>[3x]MTKRVRLSDSFNPVYPYEDESTSQHPFINPGFISPNGFTQSPNGVLTLKCLTPLTTTGGSLQLKVGGGLTVDDTNGFLKENI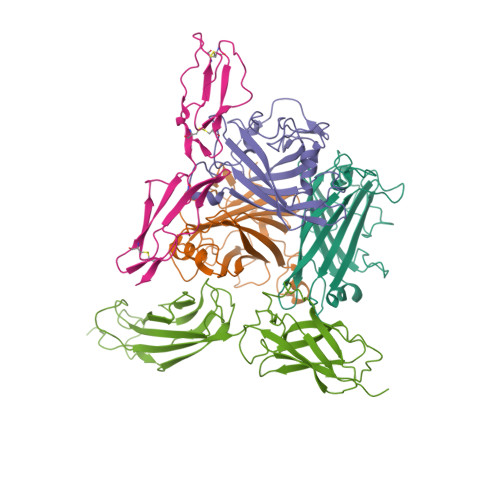SATTPLVKTGHSIGLPLGAGLGTNENKLCIKLGQGLTFNSNNICIDDNINTLWTGVNPTEANCQIMNSSESNDCKLILTLVKTGALVTAFVYVIGVSNNFNMLTTHRNINFTAELFFDSTGNLLTRLSSLKTPLNHKSGQNMATGAITNAKGFMPSTTAYPFNDNSREKENYIYGTCYYTASDRTAFPIDISVMLNRRAINDETSYCIRITWSWNTGDAPEVQTSATTLVTSPFTFYYIREDD;> MARSPGRAYALLLLLICFNVGSGLHLQVLSTRNENKLLPKHPHLVRQKRAWITAPVALREGEDLSKKNPIAKIHSDLAEERGLKITYKYTGKGITEPPFGIFVFNKDTGELNVTSILDREETPFFLLTGYALDARGNNVEKPLELRIKVLDINDNEPVFTQDVFVGSVEELSAAHTLVMKINATDADEPNTLNSKISYRIVSLEPAYPPVFYLNKDTGEIYTTSVTLDREEHSSYTLTVEARDGNGEVTDKPVKQAQVQIRILDVNDNIPVVENKVLEGMVEENQVNVEVTRIKVFDADEIGSDNWLANFTFASGNEGGYFHIETDAQTNEGIVTLIKEVDYEEMKNLDFSVIVANKAAFHKSIRSKYKPTPIPIKVKVKNVKEGIHFKSSVISIYVSESMDRSSKGQIIGNFQAFDEDTGLPAHARYVKLEDRDNWISVDSVTSEIKLAKLPDFESRYVQNGTYTVKIVAISEDYPRKTITGTVLINVEDINDNCPTLIEPVQTICHDAEYVNVTAEDLDGHPNSGPFSFSVIDKPPGMAEKWKIARQESTSVLLQQSEKKLGRSEIQFLISDNQGFSCPEKQVLTLTVCECLHGSGCREAQHDSYVGLGPAAIALMILAFLLLLLVPLLLLMCHCGKGAKGFTPIPGTIEMLHPWNNEGAPPEDKVVPSFLPVDQGGSLVGRNGVGGMAKEATMKGSSSASIVKGQHEMSEMDGRWEEHRSLLSGRATQFTGATGAIMTTETTKTARATGASRDMAGAQAAAVALNEEFLRNYFTDKAASYTEEDENHTAKDCLLVYSQEETESLNASIGCCSFIEGELDDRFLDDLGLKFKTLAEVCLGQKIDINKEIEQRQKPATETSMNTASHSLCEQTMVNSENTYSSGSSFPVPKSLQEANAEKVTQEIVTERSVSSRQAQKVATPLPDPMASRNVIATETSYVTGSTMPPTTVILGPSQPQSLIVTERVYAPASTLVDQPYANEGTVVVTERVIQPHGGGSNPLEGTQHLQDVPYVMVRERESFLAPSSGVQPTLAMPNIAVGQNVTVTERVLAPASTLQSSYQIPTENSMTARNTTVSGAGVPGPLPDFGLEESGHSNSTITTSSTRVTKHSTVQHSYS;> MEPPGRRECPFPSWRFPGLLLAAMVLLLYSFSDACEEPPTFEAMELIGKPKPYYEIGERVDYKCKKGYFYIPPLATHTICDRNHTWLPVSDDACYRETCPYIRDPLNGQAVPANGTYEFGYQMHFICNEGYYLIGEEILYCELKGSVAIWSGKPPICEKVLCTPPPKIKNGKHTFSEVEVFEYLDAVTYSCDPAPGPDPFSLIGESTIYCGDNSVWSRAAPECKVVKCRFPVVENGKQISGFGKKFYYKATVMFECDKGFYLDGSDTIVCDSNSTWDPPVPKCLKVLPPSSTKPPALSHSVSTSSTTKSPASSASGPRPTYKPPVSNYPGYPKPEEGILDSLDVWVIAVIVIAIVVGVAVICVVPYRYLQRRKKKGTYLTDETHREVKFTSL>[2x]GGHMAIEFDIQESKILKGVYIITPNKFRDLRGEIWTAFTSEAVDKLLPNGLKFIHDKFIHSKHNVIRGIHGDVKTYKLATCVYGEVHQVVVDCRKDSPTYLKHERFII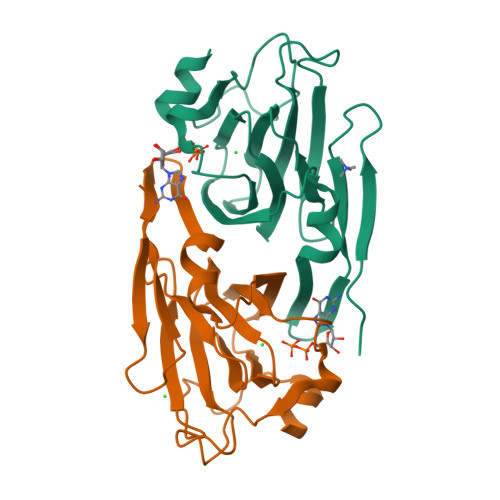NQDNQKIILVPAGFGNAHYVSSETAVYYYKCAYLGEYMDAPDQFTYAWNDERIGIDWPTNNPILSERDILAMSKDK>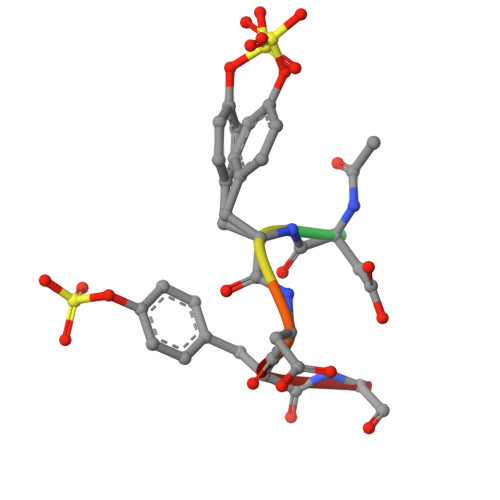 XDYDYG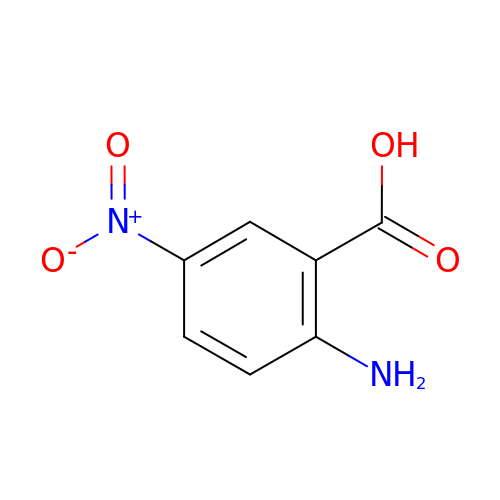5-nitroanthranilic acid | C7 H6 N2 O4 | RUCHWTKMOWXHLU-UHFFFAOYSA-N> MRAQRRFGLDLSWPRLTGVFLIDVAVLALVSHLPDAWQANHIAWWTGVGVAVLVTIVAVVTYRRTPLACALVARVLDRFVDPEMTLTEGCTPALDHQRRFGHDVVGIREYQGQLVAVVTVEGHEEAPSGRHRNRDAAPAWLPVEAVAARLRQFDVRLDAIDIVSVGTRRTSGRDDVSDVGVDDTGPVDARQPLDEHHTWLVLRMDPQRNVAAVAARDSVAATLAAATERLAHDLNGRRWTARPLTSSEIDDMDATVLAGLQPAHVRPRRRRLKYKQPEGYKEFVTSFWVSPRDITSETLERLWLPDTEATAVTVRLRPRHGGVEVSAWVRYHSSRRLRRSVWGGLNRLTGRQLDAVCASMPVPTRRPRLVVPARELHDGEELAVLV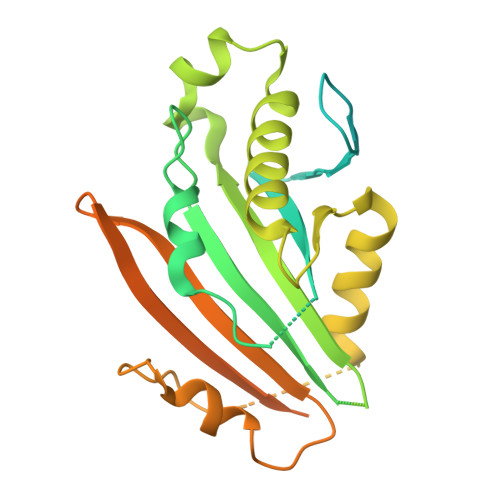GQAPAPSPSPAAAR The flavin-dependent halogenase (FDH) AetF successively brominates tryptophan at C5 and C7 to generate 5,7-dibromotryptophan. In contrast to the well studied two-component tryptophan halogenases, AetF is a single-component flavoprotein monooxygenase. A large domain tightly binds the cofactor flavin adenine dinucleotide (FAD), while the small domain responsible for binding the nicotinamide adenine dinucleotide (NADP) is unoccupied. About half of the protein forms additional structural elements containing the tryptophan binding site.

Structure determination was straightforward for non-substrate-bound (empty AetF) and 5-Br-Trp-bound AetF (AetF–5-Br-Trp). These crystals were isomorphous to each other and scaled in space groups P41 or P43 without signs of twinning or translational noncrystallographic symmetry (tNCS). Empty AetF was solved in space group P43 by molecular replacement with two molecules per asymmetric unit. AetF retained a tightly bound FAD during purification and FAD is clearly visible in all chains. Our AetF structure shows a large empty space where NADP is bound in ZvPNO and AncFMO2.

>[2x]GASGSGSGMLEVCIIGFGFSAIPLVRELARTQTEFQIISAESGSVWDRLSESGRLDFSLVSSFQTSFYSFDLVRDYEKDYYPTAKQFYEMHERWRSVYEEKIIRDFVTKIENFKDYSLISTRSGKTYEAKHVVLATGFDRLMNTFLSNFDNHVSNKTFVFDTMGDSANLLIAKLIPNNNKIILRTNGFTALDQEVQVLGKPFTLDQLESPNFRYVSSELYDRLMMSPVYPRTVNPAVSYNQFPLIRRDFSWVDSKSSPPNGLIAIKYWPIDQYYYHFNDDLENYISKGYLLNDIAMWLHTGKVILVPSDTPINFDKKTITYAGIERSFHQYVKGDAEQPRLPTILINGETPFEYLYRDTFMGVIPQRLNNIYFLGYTRPFTGGLANITEMQSLFIHKLITQPQFHQKIHQNLSKRITAYNQHYYGAAKPRKHDHTVPFGFYTEDIARLIGIHYQPNECRSVRDLLFYYAFPNNAFKYRLKGEYAVDGVDELIQKVNDKHDHYAQVFVQALSIRNMNSDEAAEWDHSARRFSFNDMRHKEGYRAFLDTYLKAYRQVENISVDDTVVDEEWNFMVKEACQVRDKVAPNIEEKTHYSKDEDVNKGIRLILSILDSDISSLPDSNGSRGSGNLKEGDRLCKFEAQSIEFIRRLLQPKNYELLFIRES> HSPLGELCPPGSHRSERPGACNRCTEGVGYTNASNNLFACLPCTACKSDEEERSPCTTTRNTACQCKPGTFRNDNSAEMCRKCSTGCPR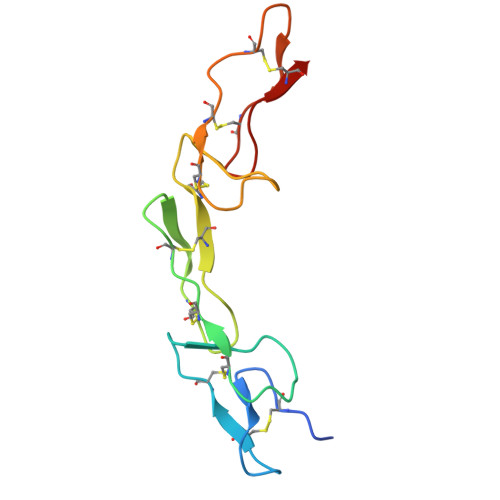GMVKVKDCTPWSDIECVHK> HHHHHHMWIGIISLFPEMFRAITDYGVTGRAVKNGLLSIQSWSPRDFTHDRHRTVDDRPYGGGPGMLMMVQPLRDAIHAAKAAAGEGAKVIYLSPQGRKLDQAGVSELATNQKLILVCGRYEGIDER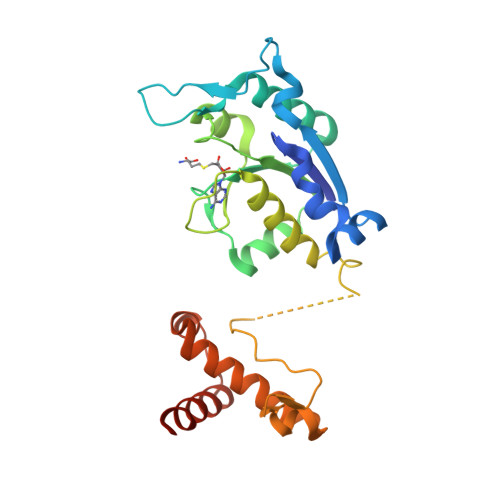VIQTEIDEEWSIGDYVLSGGELPAMTLIDSVSRFIPGVLGHEASATEDSFAEGLLDCPHYTRPEVLEGMEVPPVLLSGNHAEIRRWRLKQSLGRTWLRRPELLENLALTEEQARLLAEFKTEHAQQQHKHDGMA> SSVPGFEKLANLLKPKPGLKKLLKWADAKKPPETVFTRLRLDKTGTQLFDNTDFPVWAAYTRSVAQTDSEASAVMLKTLVSRYSDEVLSGMIAAAKKSSKTESIATKLETEQMRTWLAAKKTPDDMFLVFKLNKAGDDILSSPLLSAWTNYMKLSNKENPKAQTTLIATMTKHYGDSGVSQILAAARKSPATQSTAKRLEAEQVQLWLKKGRTPDDTFTLLSLDRAGDDLLASPQFNTWMKYINYYNKENPDEKTTVLAKLMTHFDDEELTPILVVARKVPSTESTAAKLQAEQFKNWLSADKSPEEAFTLLQLDKAGDDLLTNPQLTNWLKYTENFNLNKEINEQVTAIQVFRAQYVDDSRIANMVIAAEKVPNTQAIAKRVEDELFKGWTVVLNKPDDVFINLKLETVGENVFESPLWSFYTKFLEKYNTANPGKEQTMISGLARGYNDVTLTNMLLKAKEAPSTKTLATKLEDELVQYWLADKKLPDKLFGYLELKESVDGILTNPVFNVWLKYLNAFNDKAPVKKALMIDTLKSAFGDVAVSNMLFAAKKDPGTAKVAAT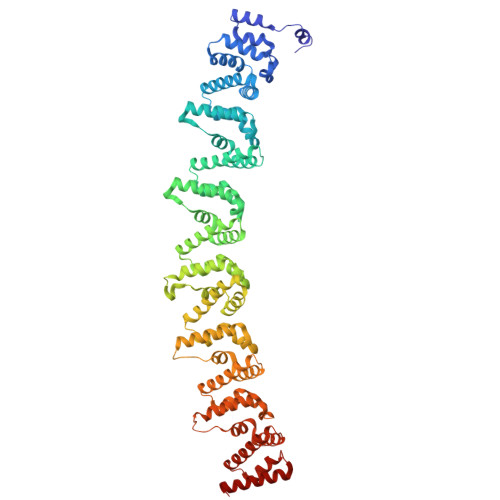LQTALLSKWVLEKKTPGQVSAILKEGAGADVSAKLLATYSAKFKVRWG>MAGKPKLHYFNGRGRMEPIRWLLAAAGVEFEEKFIGSAEDLGKLRNDGSLMFQQVPMVEIDGMKLVQTRAILNYIASKYNLYGKDIKERALIDMYTEGMADLNEMILLLPLCRPEEKDAKIALIKEKT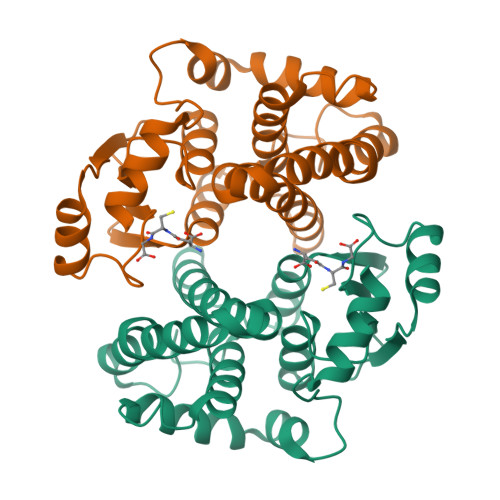KSRYFPAFEKVLQSHGQDYLVGNKLSRADISLVELLYYVEELDSSLISNFPLLKALKTRISNLPTVKKFLQPGSPRKPPADAKALEEARKIFRF[2x]>[2x]QDEKPRYKDPSVPVEERVTDLLGRMTLEEKMSQLIQGDITNWMNETTGEFNLTGLEWSTKMRGGMFYV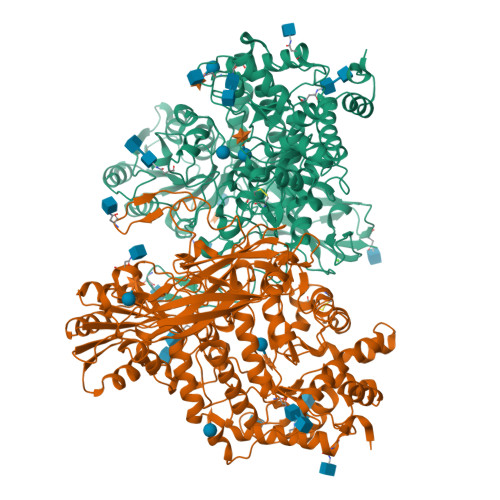GYPVPWDYIADNVKKAQDYILQNTTLGIPAIVQTESLHGFLIGNATIYNSPIGFACSFNPELIEKMARLIGQEASALGVNHVMGPVVDLARELRFGRVEETYGEDPFLAGEIGYHYTKGIQSHNISANVKHFVGFSQPEQGLNTAPVHGGERYLRTTWLPSFKRAIMDAGAWSIMSAYHSYDGIPAVADYHTLTEILREEWGYKYWVTSDAGASDRVCTAFKLCRADPIDKEAVTLAILPAGNDVEMGGGSYNFETIIDLVNAGKLDIEIVNTAVSRVLRAKFEMGLFENPYNAAPASEWNKLIHTQEAVDLARELDRESIVLLENHDNALPLKKSGSIAVIGPMAHGFMNYGDYVVYESQYRGVTPLDGIKAAVGDKATINYAQGCERWSNDQSGFAEAVEAAKKSDVAVVVVGTWSRDQKELWAGLNATTGEHVDVNSLSLVGAQAPLIKAIIDTGVPTVVVLSSGKPITEPWLSNNTAALVQQFYPSEQGGNALADVLFGDYNPSGKLSVSFPHSVGDLPIYYDYLNSAREIGDAGYIYSNGTLEFGHQYALGNPKAWYPFGYGKSYSSFEYGAVKLDKTNVTEADTVTVSVDVKNTDATREGTEVVQVYVVDEVASVVVPNRLLKGFKKVVIPAGQTKTVEIPLKVQDLGLWNVRMKYVVEPGAFGVLVGSSSEDIRGNATFYVQVDHHHHHH> GQYKDNIRHGVCWIYYPDGGSLVGEVNEDGEMTGEKIAYVYPDERTALYGKFIDGEMIEGKLATLMSTEEGRPHFELMPGNSVYHFDKSTSSCISTNALLPDPYESERVYVAESLISSAGEGLFSKVAVGPNTVMSFYNGVRITHQEVDSRDWALNGNTLSLDEETVIDVPEPYNHVSKYCASLGHKA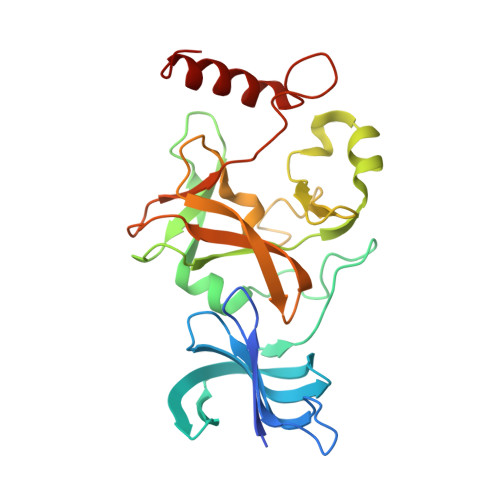NHSFTPNCIYDMFVHPRFGPIKCIRTLRAVEADEELTVAYGYDHSPPGKSGPEAPEWYQVELKAFQATQQK>SIPGQVADQAPLPSLAPMLEKVLPAVVSVRVEGTASQGQKIPEEFKKFFGDDLPDQPAQPFEGLGSGVIINASKGYVLTNNHVINQAQKISIQLNDGREFDAKLIGSDDQSDIALLQIQNPSKLTQIAIADSDKLRVGDFAVAVGNPFGLGQTATSGIVSALGRSGLNLEGLENFIQTDASINRGNAGGALLNLNGELIGINTAILAPGGGSVGIGFAIPSNMARTLAQQLIDFGEIKRGLLGIKGTEMSADIAKAFNLDVQRGAFVSEVLPGSGSAKAGVKAGDIITSLNGKPLNSFAELRSRIATTEPGTKVKLGLLRNGKPLEVEVTLDTSTSSSASAEMITPALEGATLSDGQLKDGGKGIKIDEVVKGSPAAQAGLQKDDVIIGVNRDRVNSIAEMRKVLAAKPAII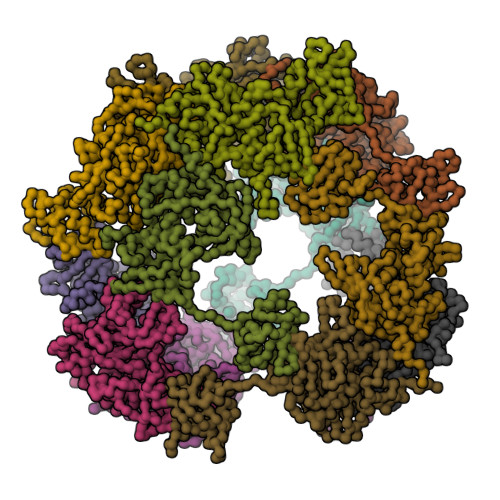ALQIVRGNESIYLLMRLEHHHHHH[12x]> LRQCLPCGPGGKGRCFGPSICCGDELGCFVGTAEALRCQEENYLPSPCQSGQKPCGSGGRCAA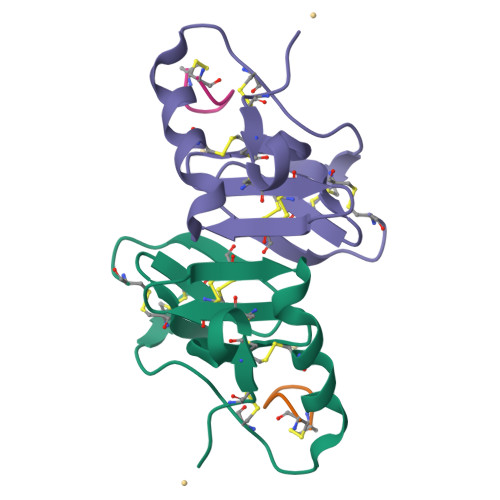AGICCNDESCVTEPECREGVGFPRRV;> CYFQNCPKG> QDKCKKVYENYPVSKCQLANQCNYDCKLDKHARSGECFYDEK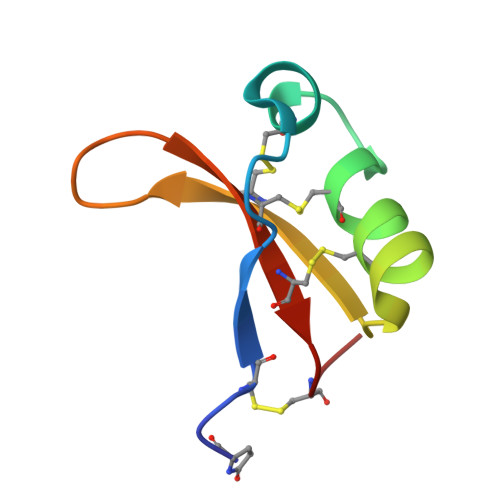RNLQCICDYCEY>MVRERTFIAVKPDGVQRGLIGEIIKRFEAKGFKLAGMKYIQASEDLLKQHYIDLADKPFYPGLCKYMSSGPVVAMCWEGTGVVKTARVMMGETRPADSKPGTIRGDFCIEVGRNIIHGSDSVESANKEIALWFKPEELV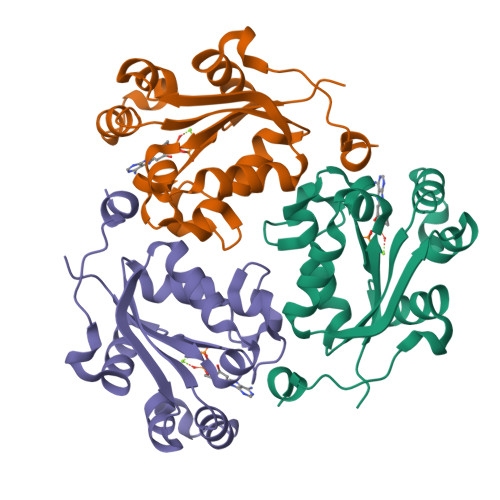SWTQTNESWIYE[3x]>[2x]MKLIVVTTPTFFVEEDKIITALFEEGL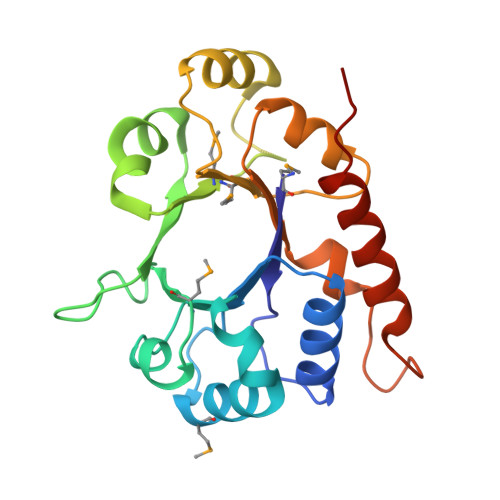DILHLRKPETPAMYSERLLTLIPEKYHRRIVTHEHFYLKEEFNLMGIHLNARNPSEPHDYAGHVSCSCHSVEEVKNRKHFYDYVFMSPIYDSISKVNYYSTYTAEELREAQKAKIIDSKVMALGGINEDNLLEIKDFGFGGAVVLGDLWNKFDACLDQNYLAVIEHFKKLKKLADLEHHHHHH Here, we describe the design, characterization, and application of de novo helical hairpins that heterodimerize to form 4-helix bundles in cells. Starting from a rationally designed homodimer, we construct a library of helical hairpins and identify complementary pairs using bimolecular fluorescence complementation in E. coli. We characterize some of the pairs using biophysics and X-ray crystallography to confirm heterodimeric 4-helix bundles. Finally, we demonstrate the function of an exemplar pair in regulating transcription in both E. coli and mammalian cells.

We attempted to crystallize all four selected pairs and were successful with 26α/26β. The 26α/26β complex formed the targeted heterodimer of hairpins, which was confirmed as a 4-helix CC with knobs-into-holes packing using the program Socket2.51 The heterodimer has a syn topology. This is different to the parent CC-HP1.0 structure, which crystallized in an anti conformation. However, the syn conformation is consistent with the designed charge patterning of CC-HP1.0 as depicted in the helical wheels for the design, and with AlphaFold2 predictions. Moreover, although the anti and syn forms are likely close in energy, and the linkers in the split-YFP assay should be flexible enough to allow both topologies, we suggest that the syn arrangement is favored. In contrast, near-complete quenching occurred when 26β-c4CF and 26α-nMSE were mixed, demonstrating the proximity of the 4CF and MSE residues. These data are consistent with 26α/26β forming a heterodimer with a syn topology in solution as observed in the experimental X-ray crystal structure. In summary to this section, the in vitro solution-phase biophysical data confirm that the cognate pairs selected from the in vivo BiFC assay, i.e., 9α/9β, 14α/14β, 21α/21β, and 26α/26β,all form stable, helical heterodimers consistent with the targeted 4HB structures. At the lowest concentration of peptides that gave measurable CD spectra (i.e., 1 μM total peptide), second derivatives of melting curves returned melting temperatures of 43 °C for 26α, 30 °C for 26β, and 48 °C for the mixture 26α/26β. This suggests that the 26α/26β heterodimer should be well formed and stable, whereas the individual peptides should be unfolded or partially folded at concentrations close to those anticipated in cells and at the required temperature for cell experiments (37 °C).

>[4x]XGELEALAKKTKALTWKFKALSKEPSAQELEALTQECEALGKKLKALAQGX;>[4x]XGELEALGKKFKALAWKVKALSKEPSAQELEALTQEAEALGKKIKALAQGX Among bisindoles, reductasporine is distinct due to its dimethylpyrrolinium structure. Its previously reported biosynthetic gene cluster encodes two unique tailoring enzymes, the imine reductase RedE and the dimethyltransferase RedM, which were shown to produce reductasporine from a common bisindole intermediate in recombinant E. coli. RedE reduces compound 4 to didemethylreductasporine, and then RedM catalyzes two methylations to give reductasporine. RedM is a homodimeric protein with monomers consisting of a largely α-helical N-terminal domain (α1-10, β1-3) and a Rossmann-like fold C-terminal domain (α12–16, β4-10) bridged by a long interdomain α-helix (α11). The C-terminal domain possesses a Rossmann-like fold typical of Class I SAM-dependent methyltransferases, with a β-sheet of five parallel strands terminated with two antiparallel strands each interspersed with α-helices.

Between the RedM-SAH and RedM-SAM binary complexes, there are distinct open and closed conformations, respectively. The homodimers of both unliganded-RedM and RedM-SAH structures superpose well on each other (rmsdCα = 0.175 Å, 553 Cα) and comparatively poorly upon the RedM-SAM homodimer (rmsdCα = 1.244 Å, 593 Cα) due to a substantial displacement of the C-terminal Rossmann-like SAM-binding domain. Lastly, Chain B of the RedM-SAH complex and unliganded-RedM chain A have slightly rotated Rossman-like domains compared to their dimer partners with an average Cα displacement of 1.8 Å between each pair. The cofactor binding pocket is outlined by the C-terminal ends of β4-8 and clear electron density shows the cofactor is held in an extended conformation similar to related small molecule methyltransferases. The main chains of C185, A186, and G188 form the foundation of the cavity between the ribosyl and methionine moieties, while D182 hydrogen bonds to two conserved water positions creating the basis for a network of hydrogen bonds bridging the α-amine to I183, Y280, and G249 via its amide nitrogen. The carbonyl groups of G184 and G249 receive hydrogen bonds from the α-amine, while H250 and Y280 donate hydrogen bonds to the cofactor carboxylate group. The ribosyl hydroxyl groups interact closely with D207, representing the second conserved binding motif in SAM-dependent methyltransferases. The adenine ring is clamped between F235 and L208 and capped with a hydrogen bond to D234. Docking search with 3 on the open conformation places moderately favorable poses at the junction of helices α7, α11, α15, and α′1 and αʹ2 of the dimer partner, an average of 20 Å away from the bound SAH cofactor. D15 may be engaged in a salt bridge to R163 joining the N-terminus to the interdomain helix (α11); however, this interaction only has unambiguous electron density in one monomer of the RedM-SAH complex.

>[2x]MSDTSPGPEHAPAIDRLLQIATGFMASKVLLVAASLGLFTELAAGPLRGEELRARLRLHPRSARDFFDTLVALGVLERTNGAYANTPATAQYLVRGKSAYLGGLLEMSDARMYELWGRLDEGLRTGNPQNEIRTGEEGIYATLYDDPDRLDAFQQAMTGLSMRSAHALAEAIDWSAYRTVADIGCAEGTVLIHLLERHPHLRGTGFDLAAVRPSFQRRHEESGLGDRLAFRAGDFFAEPLPQADALVFGHILSNWALPKAKTLLRKAHEALPEGGIVVIYETLIDDERRENVPGLLMSLTMLLETPGGFEYTGADCREWLADAGFRESRVQYLAGPESMVIATK>MHHHHHHMFSRFSNVVSEIEKKYVDKISISEIMTKAIEGLLSNLDAHSAYLNEKKFKEFQAQTEGEFGGLGITVGMRDGVLTVIAPLEGTPAYKAGVKSGDNILKINNESTLSMSIDDAINLMRGKPKTPIQITIVRKNEPKPLVFNIIRDIIKLPSVYVKKIKETPYLYVRVSGFDKNVTKSVLEGLKANPKAKGIVLDLRGNPGGLLNQAVGLSNLFIKEGVLVSQKGKNKEESLEYKANGRAPYTNLPIAVLVNGGSAAASEIVAGALQDHKRAVIIGEKTFGAGSVAMLLPVNKDEAIKITTARYYLPSGRTIQAKGITPDIVIYPGKVPENENKFSLKEADLKHHLEQELKKLDDKTPNSKEADKDKKNEEEKEVTPKMINDDIQLKTAIDSLKTWSIVDEKMDEKAP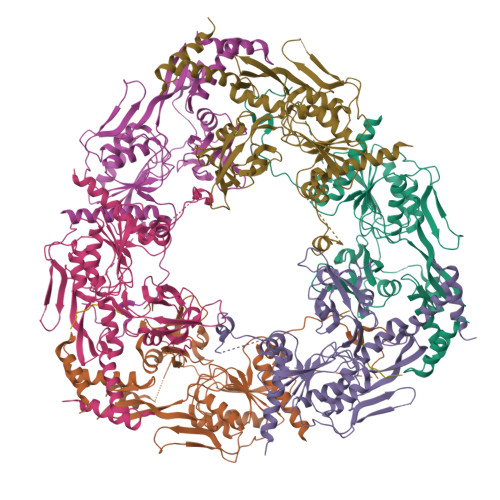KKK[6x]>GPLGSKEQGVVRKAGWLFFKPLVTLQKERKLELVARRKWKQYWVTLKGCTLLFYETYGKNSTEQNSAPRCALFAEDSIVQSVPEHPKKEHVFCLSNSCGDVYLFQATSQTDLENWV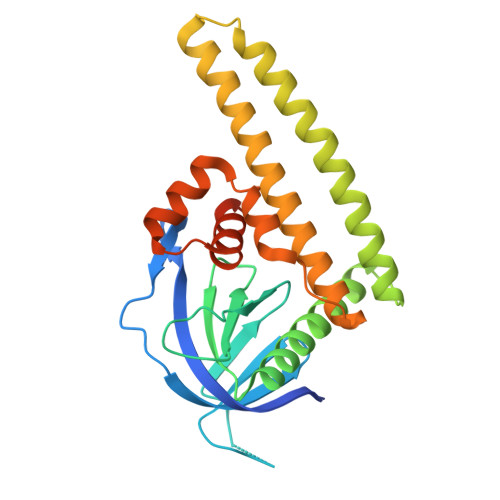TAIHSACASLFAKKHGKEDTVRLLKSQTRSLLQKIDMDSKMKKMAELQLSVVSDPKNRKAIENQIRQWEQNLEKFHMDLFRMRCYLASLQGGELPNPKSLLAATSRPSKLALGRLGVLSVSSFHALVCSRDDSTLRKRTLSLTQRGK[4x]>[2x]MITFIGHVSKDVNVVDGKREI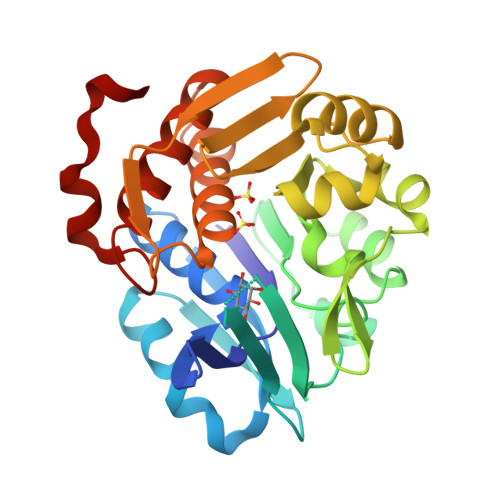AYGGGVVMGAITSSLLGVKTKVITKCTREDVSKFSFLRDNGVEVVFLKSPRTTSIENRYGSDPDTRESFLISAADPFTESDLAFIEGEAVHINPLWYGEFPEDLIPVLRRKVMFLSADAQGFVRVPENEKLVYRDWEMKEKYLKYLDLFKVDSREAETLTGTNDLRESCRIIRSFGAKIILATHASGVIVFDGNFYEASFRSWSLEGRTGRGDTCTAAFLVGFVFKKMSIEKATKFAAAVTSVKMRHPGPLRREDLEAISGDQYF> MWEANELSSTNTFSHQAEMDWPSANWWQRYQDAQLNHLIEEALQHSPSLCMAMARLKGAQGFARQAGAIRSFDLGLAASATESKVSERYQSATPPDGWNDYGTLTLNFQYDFDFWGKNRAAVVAATSELAAAEAESVAARLMISTSIANAYAELARLYANQETVHAALQVRNKTVELLEKRYANGLETLGSVSQAKAVAASVEAELLGIQESIQLQKNALAALVGQGPDRAASIEEPHITLTSRYGLPSEAGVGLLGHRADITAARWRAEAAAQQVGIAQAQFYPDVTLSAFIGYQAFGLDHLFDSGNDAGAIGPAIYLPLFTGGRLEGQLTSAEARYQEAVAQYNGTLVQALHEIADVVTSSQA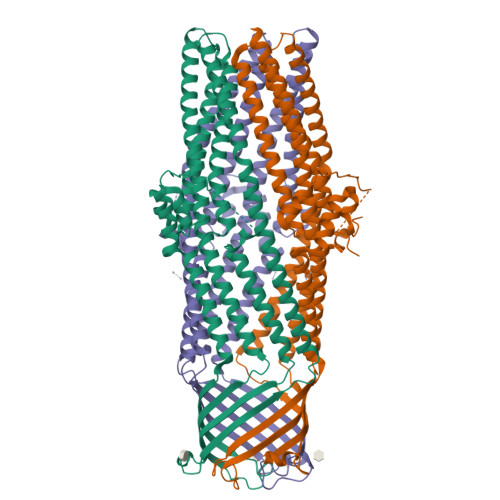LQARINKTEQAVQQAEQALHIATNRYQGGLATYLDVLVAEESLLNNQRALVNLQSRAFSLDLALIHALGGGFETTES>AYRDQPLGELALSIPRASALFRKYDMDYAAGGKQTLARAAARKELDVEVIEAELAKLAEQPIEKDWRSAPLAEIIDHIIVRYHDRHREQLPELILQATKVERVHADKPSVPKGLTKYLTMLHEELSSHMMKEEQILFPMIKQGMGSQAMGPISVMESEHDEAGELLEVIKHTTNNVTPPPEACTTWKAMYNGINELIDDLMDHISLENNVLFPRALAG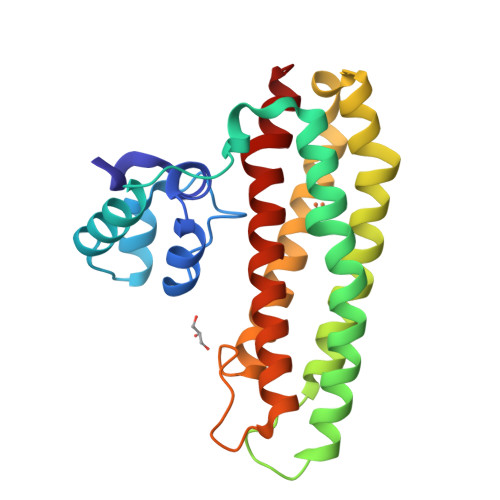E[2x]> MAQRGIREYDAKNLLARYLPEYLDDFSYKGNLALVGPETDIEGLEAENPWLKTTRLVVKPDQLFGKRGKLGLVLLDADWEEAKEYLNEKMGLEVTIGGITGRLSYFLIEPFTPHKEEYYVAISSDYEGDNIFFSMDGGVGVEENWEKVISIHVDSLEGIDALDVGSKLPAELGDKRALVEEFITALWRFYSDTGFAYVEINPFTFSGRGIVPLDMVAKLDDAEEYWQKKRWSELAFPEPFGRTPSKEELFIKEIDSKTGASLKLTILNPEGRVWTMVAGGGASVIYADTICDLGHADEMANYGEYSGDPNTEETYHYTCTILDLMTRSKNPNGKVLLIGGAIANFTDVAKTFKGVVMALEEYQQKLQEADIEIYVRRGGPNYEQGLKLMRDLGKRLGVPIQVHGPETHMTRIVPLALEENQ;> MSRKDYVLFDINTKAFVYGYQTNAIQRMLDFDYVCKRSSPSISAIINPSRAGIHKAFWGTKEIILPMYKTIPLAALAYPEADVMVNFASHRSAFETTMEALKEDTIRIVAVIAEGVPERQSRVMAATARKLDKIVIGPATVGGMTAGAFRIGNTAGTIENIIASKLYRPGCVGFVSKSGGMLNEAFNIISRNSDGIYEGVAIGGDRYPGSNMLDHILRYERNPAIKMIACLGELGGEDEYMIIQALKEKKITKPLVAWVTGTCSPYLPASVQFGHAGAKANTEKETAQAKNDAFRQAGAYVPRSFDDYGEMVRQVYDML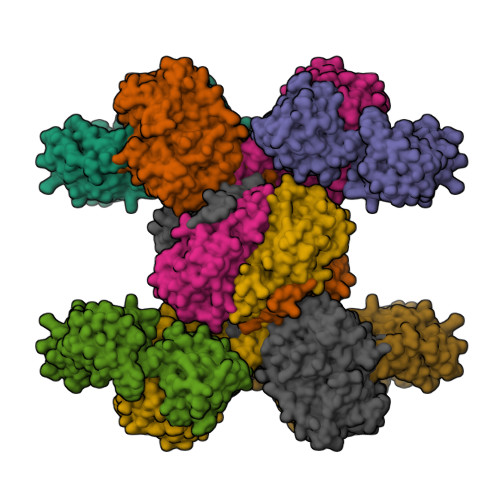LTRGIVQKFDEPEVPRIPTDYSKALATGDIRKPTTFICTISDDSGEELLYAGKKLSDVLDRKMGIGGVIGLLWFKKELPEYAAHFIELVIQIVADHGPAVSGAHNAIVASCAGKDLISSLCSGLLTIGPRFGGAIDDAAREFKRAQETGLAPEQFVGEMKKKGINIPGIGHKIKSVKNPDKRVQLLISYARANFPSTELLNYALQVEELTTAKKGNLILNVAGCIGILFIDLMSSCGAFSKEEIDEVVRLGYLNGLFALGRSIGLIGHILDQKRLGSRLYRHPAEDIAYMMPSEEEIQCKRDRGGSHHHHHH>[5x]QEEGEDNGGEDNKKLRGALSSAILSEKPNVKWEDVAGLEGAKEALKEAVILPVKFPHLFKGNRKPTSGILLYGPPGTGKSYLAKAVATEANSTFFSVSSSDLVSKWMGESEKLVKQLFAMARENKPSIIFIDEVDALTGTRGEGESEASRRIKTELLVQMNGVGNDSQGVLVLGATNIPWQLDSAIRRRFERRIYIPLPDLAARTTMFEINVGDTPCVLTKEDYRTLGAMTEGYSGSDIAVVVKDALMQPIRKIQSATHFKDVSTEDDETRKLTPCSPGDDGAIEMSWTDIEADELKEPDLTIKDFLKAIKSTRPTVNEDDLLKQEQFTRDFGQEGN

The large and diverse family of AAA+ ATPases (ATPases Associated with various Activities) includes multiple members that form hexamers and are believed to unfold protein substrates by translocating them through their central pore. The structures of several AAA+ ATPases have been determined by electron cryo-microscopy (cryo-EM) in the presence of engaged substrate, including the mitochondrial inner membrane protease YME1, the disaggregase Hsp104, the chaperone ClpB, the TRIP13 mitotic checkpoint regulator, the SNARE disassembly machine NSF, the VAT archaeal homolog of Cdc48/p97, the proteasome, and Vps4, which associates with the positive regulator Vta1 to drive the ESCRT pathways that mediate multiple membrane fission events in eukaryotic cells by disassembling filaments comprised of ESCRT-III subunits. Here, we show that the mechanism proposed for linear, extended polypeptides is also compatible with translocation of more complex substrates. Structure determination showed that a primary segment of the circular peptide binds indistinguishably from the isolated linear peptide, while a secondary segment packs against it in a β-ladder hairpin configuration that passes through the hexamer pore without distorting the Vps4 structure or making intimate contacts with Vps4. These observations indicate that AAA+ ATPases can translocate two chains of a substrate, such as would occur in crosslinked chains or in ubiquitin conjugates, using the same mechanism as for an extended polypeptide.

Because other regions of the cF30 and cFF30 reconstructions are essentially identical, we used particles from both datasets to reconstruct a combined map at 3.6 Å. The overall structure superimposes closely with the previously reported linear peptide complex, including the same helical arrangement of five Vps4 subunits (subunits A-E). Although details of nucleotide configuration are not definitively resolved, consistent with the earlier structure, the subunit AB, BC, and CD interfaces appear to bind ADP·BeFx (ATP), while the DE interface density is ambiguous, but could be ADP or an ADP/ADP·BeFx mixture. The density and refined models for the cF30 and cFF30 peptides are essentially identical, with two polypeptide strands passing through the Vps4 pore. The pore loop positions and the substrate strand with the strongest density (primary strand) superimpose closely on the earlier peptide F complex structure, except that density for the peptide now extends both N-terminally and C-terminally for two additional residues. The density is consistent with the peptide F sequence binding in the same register as the earlier peptide F complex, with odd-numbered residues binding to an array of class I pockets and even-numbered residues binding to an array of class II pockets. The returning strand of the circular peptides has weaker density, indicating that it is more mobile.> MKPTTVIGAGFGGLALAIRLQAAGIPVLLLEQRDKPGGRAYVYEDQGFTFDAGPTVITDPSAIEELFALAGKQLKEYVELLPVTPFYRLCWESGKVFNYDNDQTRLEAQIQQFNPRDVEGYRQFLDYSRAVFKEGYLKLGTVPFLSFRDMLRAAPQLAKLQAWRSVYSKVASYIEDEHLRQAFSFHSLLVGGNPFATSSIYTLIHALEREWGVWFPRGGTGALVQGMIKLFQDLGGEVVLNARVSHMETTGNKIEAVHLEDGRRFLTQAVASNADVVHTYRDLLSQHPAAVKQSNKLQTKRMSNSLFVLYFGLNHHHDQLAHHTVCFGPRYRELIDEIFNHDGLAEDFSLYLHAPCVTDSSLAPEGCGSYYVLAPVPHLG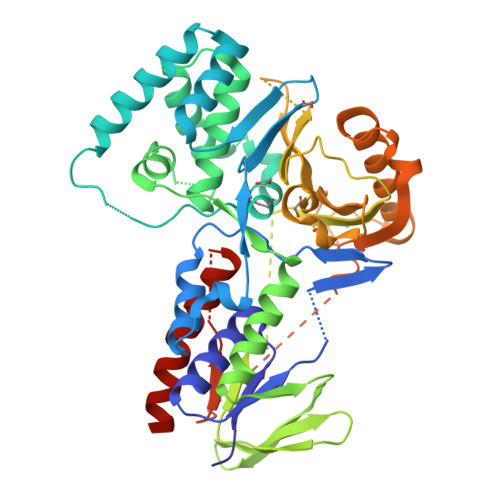TANLDWTVEGPKLRDRIFAYLEQHYMPGLRSQLVTHRMFTPFDFRDQLNAYHGSAFSVEPVLTQSAWFRPHNRDKTITNLYLVGAGTHPGAGIPGVIGSAKATAGLMLEDLIGGSHHHHHH2-(2-CHLORO-PHENYL)-5,7-DIHYDROXY-8-(3-HYDROXY-1-METHYL-PIPERIDIN-4-YL)-4H-BENZOPYRAN-4-ONE 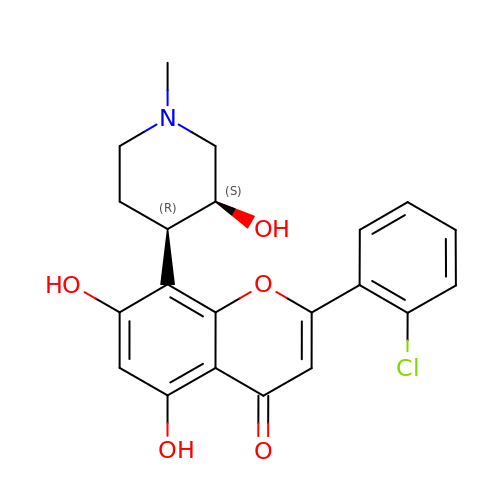| C21 H20 Cl N O5 | BIIVYFLTOXDAOV-YVEFUNNKSA-N The first committed step toward l-phenylalanine and l-tyrosine is the conversion of chorismate to prephenate, catalyzed by chorismate mutase (CM). In M. tuberculosis, CM (MtCM, a dimer encoded by Rv0948c, aroQδ) has evolved to transiently interact with DS (MtDS, a tetramer encoded by Rv2178c, aroG) to form a heterooctameric complex. MtCM represents the structurally simple AroQδ subclass of CMs composed of two intertwined three-helix subunits. Only the complexed, but not the free dimeric MtCM, is responsive to feedback regulation by Phe and Tyr.

To elucidate the structural basis for the boost in catalytic activity, we solved the crystal structure of the top variant N-s4.15 to 1.5 Å resolution. In N-s4.15, this loop adopts a similar conformation as in EcCM, *MtCM, and MtDS-complexed MtCM that is distinct from the loop conformation in free MtCM. The activated loop is highly kinked, either because of Pro52 in the evolved variant or induced by binding to MtDS. Asp55 ensures the return to the helical conformation at the C-terminal side of the H1-H2 loop by N-capping helix H2. Interestingly, the Asp55 side chain of N-s4.15 engages in a hydrogen bond with Arg18 from the other protomer across the active site, a catalytic residue that aligns well with the corresponding active conformation in the MtDS complex. The crystal structure of N-s4.15 shows that Pro87 introduced another kink, resulting in reorientation of the C terminus. However, in the variant N-s4.15, the C-terminal residues are less well-ordered compared with MtDS-activated WT MtCM (average B-factors of Pro87 and Asp88 are >100 Å2), and beyond residue 88, hardly any electron density is visible, suggesting that the C terminus is flexible in solution. Whereas the guanidinium group of Arg46 in the evolved N-s4.15 is still not in an ideal position but is pulled toward the newly introduced acidic residue Asp55, it is more similar to that of MtDS-activated MtCM compared with native uncomplexed MtCM. Overall, most active site residues of N-s4.15 adopt conformations resembling the ones observed in the MtDS-activated WT MtCM. The crystal structure of N-s4.15 implies that its improved activity is due to a combination of pre-positioning active site residues for efficient substrate and transition state binding, tighter packing of the active site, and an overall stabilization of the fold, as reflected by the increase in the enzyme's melting temperature.

> MNLEMLESQPLPEIVTLREEIDRLDAEILALVKRRAEVSQAIGKARMASGGPRLDHSREMKIIERYSELGPVGKDLAILLLRLGRGPDAM> ETVQVNLPVSLEDLFVGKKKSFKIGRKGPHGASEKTQIDIQLKPGWKAGTKITYKNQGDYNPQTGRRKTLQFVIQEKSHPNFKRDGDDLIYTLPLSFKESLLGFSKTIQTIDG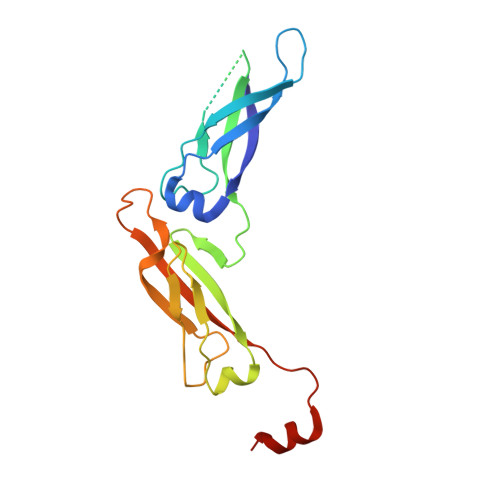RTLPLSRVQPVQPSQTSTYPGQGMPTPKNPSQRGNLIVKYKVDYPISLNDAQKRAIDENF> MEHVAFGSEDIENTLAKMDDGQLDGLAFGAIQLDGDGNILQYNAAEGDITGRDPKQVIGKN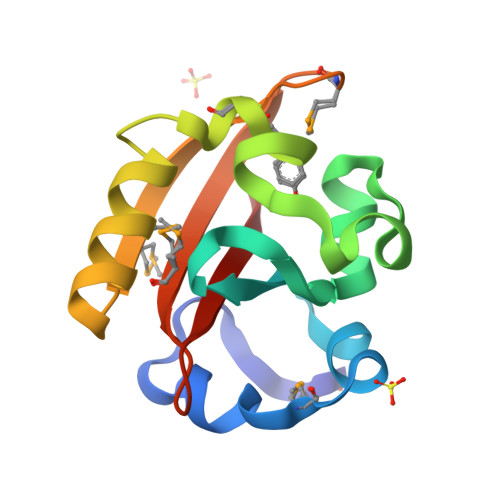FFKDVAPCTDSPEFYGKFKEGVASGNLNTMFEYTFDYQMTPTKVKVHMKKALSGDSYWVFVKRV>MSGGLEVKNFDFKVGKFLTVGGVINNYAKRFSINVGESTNSLSLHLDHRFNYGADQNTIVLNSMVNSGWETEQR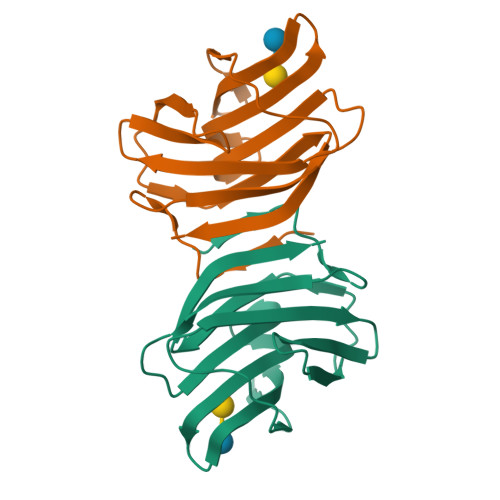SKNFPFSAGEYFEITITFDTNKFYIELLDGHKLEFPNRYKKEALNFLSLAGDARLTFVKLE[2x]> MEINRAEIRREITRYTGLIEQQTQLNISDNDENILKTLIADYNLRMRRDALLGELARLDELRDISQVKGVEYKVTIPLLPVISTLNQHEFEITQANIETDFIADNVTFVTSFVPADLDLEQTIQRVFFRTTATTPHFQSFNLVIEILNYDQDSGDVELHVKIMIVRPNSDVVNYDYTWIGKDYERISVCYNLISHLQRIDGPHGRDDEAEMPIYRIIRRDSGSIPSYASGEHLYVISSHLHVDEIVRRREHKSISVDVTQLSLILPIIRTFNPVDLREVRIEDITPGIEFTINMEVSTYLAESSGSHVDMQRAIMNHADKIVGNYTGQQWNVQSNMLSEVRTQMLEEEDEEARQRGDYTTSTLVQTMAQVSDLFSSTILYRRAEARLDNTVGAFELLRPVLSIPSEYVHNGRVGPITNIPANASIVTSSSSGAGQVRNIFKPIGDQTINESHFANVFSNDEYAIYLRFSYRQAPVQSETVYLQQNLPSMRIVSPSSVSTTVSTAVIGGNTIHINCPIRPHREDRLVSGGVQVPRQSTAVEIRVQEILIGYRQATTFPIDTEGRLSLELMYGLESRSAVGNTMSPVRFVTVNDGEFFGLTCPIDLTLSTVVDPSSYLSDGVILVATAFEDLRGYAWVATLGGDWPRTYNSSMRAFNVLTGGDINLSTEYGSEMTYTFKVELPIVYMFNNMTVISNNVPRVPVLGVTYASIYQDSRTELEARRFLQTLVFRIHGNWSARIPYTPGNLPTRNTANQHQDIQQVINDSISQELGRLSDELLNM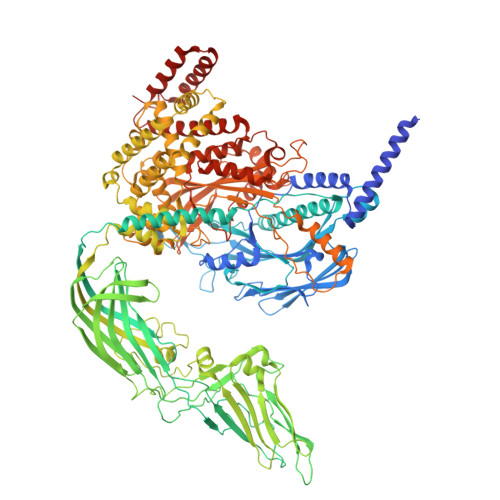KNRLDHLERQFEMFIQSQESEWWEILLNVVMDTVLGYFSTFAGNALKSAQQAISKAVGYTRRVLMTVTKTMRNGPIFTRLLGAKNLSGQALASLETLVESVLRSINVKKSRFMSGAEPLYKNNKVAQHIDNTEKMNMMMDFSFANRNNRQNITADTLSRMHTQNAHGTSDTVLPAMRVYYRPLGFLDKRVGEALHKGITRPEALKKQLRSDVANVGTRAPSHAFMTYTDVLYEDAGSYIVSKRYLGIGELNRFGRTTSDKNADIGGVNIKYRVNKITADGKYIIDRLSHTESGYTAADVDRLYRSLFGKQGDGLSTEQKWMDISRGVDAKIISADMVSEEFLSSKYTGQMIDELINSPPQFNYSLIYRNCQDFVLDVLRVAQGFSPSNKWDVSTAARMQQRRVISLMDDLMSESETFARSAHSNHSLLQQIRRSYVKARKRGDLHTVKALQLRLKGFFQI> GIIVSNPTELIKQGEQLEQMAQQLEQLKSQLETQKNMYESMAKTTNLGDLLGTSTNTLANNLPDNWKEVYSDAMNSSSSVTPSVNSMMGQFNAEVDDMTPSEAIAYMNKKLAEKGAYDRVMAEKAYNNQMQELSDMQA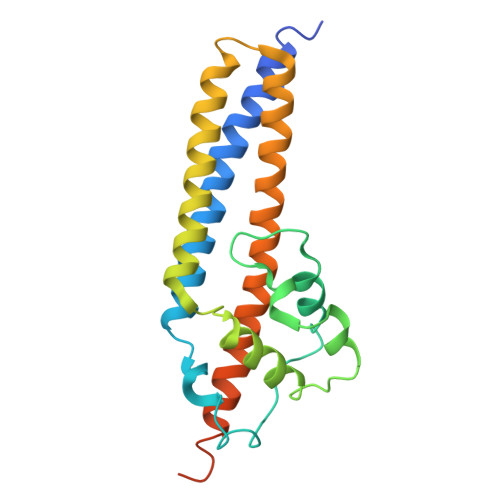LTEQIKSTPDLKSIADLQARIQTSQGAIQGEQAKLNLMNMLQQSQDKLLRAQKDRATRNFVFGTGGDVTASPSIN> GSDGWTCAGSDFDGDQVRGQARHWVDQQKTKFSDFQTHDGVQLCHFELGEGNQ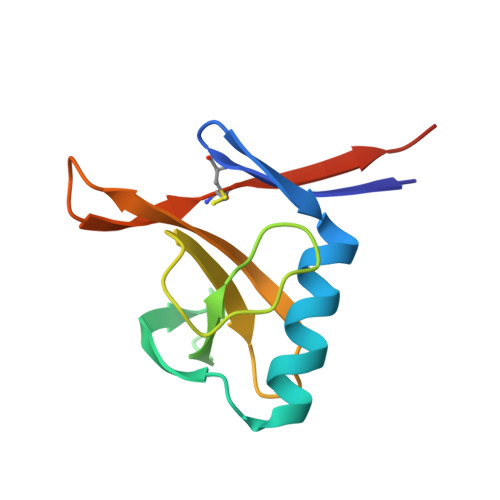LTQSFTGFRAYCDEPGDVYNVRYWDVSSRTWVLCTHYDIDFESDYR> MENGYTYEDYKNTAEWLLSHTKHRPQVAIICGSGLGGLTDKLTQ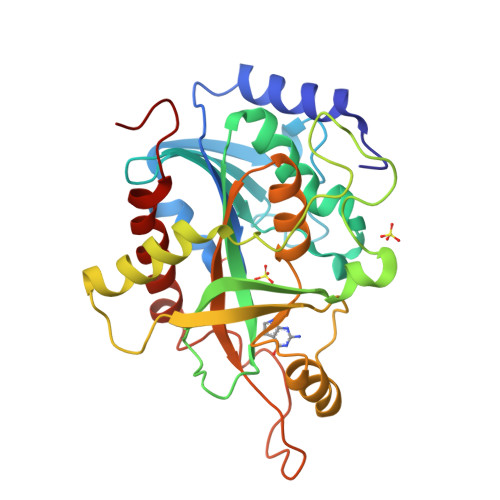AQIFDYSEIPNFPRSTVPGHAGRLVFGFLNGRACVMMQGRFHMYEGYPLWKVTFPVRVFHLLGVDTLVVTNAAGGLNPKFEVGDIMLIRDHINLPGFSGQNPLRGPNDERFGDRFPAMSDAYDRTMRQRALSTWKQMGEQRELQEGTYVMVAGPSFETVAECRVLQKLGADAVGMSTVPEVIVARHCGLRVFGFSLITNKVIMDYESLEKANHEEVLAAGKQAAQKLEQFVSILMASIPLPDKAS>MYKDFANFIRTNKKDLLNNWMNEMEKQSDPLINDIAKEPMYEETSIEFVDLIVSNITENGSKFNEKLDDFAEKVVHLGWPIHFVTTGLRVFGLLVYTAMRDEDLFLKREEKPEDDAYYRFETWLSSMYNKVVTAYADTWEKTVSIQKSALQELSAPLLPIFEKISVMPLIGTIDTERAKLIIENLLIGVVKNRSEVVLIDITGVPVVDTMVAHHIIQASEAVRLVGCQAMLVGIRPEIAQTIVNLGIELDQIITTNTMKKGMERALALTNREIVEKEG[40x];>MGIPILKLGECLLISIQSELDDHTAVEFQEDLLAKIHETSARGVVIDITSIDFIDSFIAKILGDVVSMSKLMGAKVVVTGIQPAVAITLIELGITFSGVLSAMDLESGLEKLKQELGE[20x]

The stressosome is a pseudo-icosahedral megadalton bacterial stress-sensing protein complex consisting of several copies of two STAS-domain proteins, RsbR and RsbS, and the kinase RsbT. Upon perception of environmental stress multiple copies of RsbT are released from the surface of the stressosome. Free RsbT activates downstream proteins to elicit a global cellular response, such as the activation of the general stress response in Gram-positive bacteria. The activation state of the stressosome is reset by the removal of phosphates from RsbS and RsbR by the phosphatase RsbX, allowing for a new round of phosphorylation.

Here, we determined a 3.87 Å reconstruction from a D2 symmetrized cryo-EM map of the stressosome of Listeria innocua (LiRsbRS) assembled from co-expressed LiRsbR and LiRsbS proteins. The stoichiometry of RsbR:RsbS was identical to the one described for the Bacillus stressosome, 20 LiRsbR2:10 LiRsbS2. The 10 LiRsbS dimers form two hook-shaped strips along the core (f in yellow and orange color). A pentameric plane thereby comprises five triangular faces, all of them consisting of one RsbS and two RsbR dimers. LiRsbR enters the STAS domain as the linker helix (ɑ0), while a beta-strand (β0) is found at the N-terminal end in LiRsbS. ɑ3 is well-resolved in LiRsbRS, while it is not resolved in LmRsbR. Interestingly, the MS analysis on the phosphorylation state of the SEC fraction used for structure determination revealed a phosphorylation of Thr241, while conserved sites Thr175 and Thr209 were not phosphorylated. Close to Thr241 in LiRsbR, a spherical density was assigned as phosphoryl group in accordance with the ESI–MS–MS. The phosphoryl-group brings Thr241 in interaction range to Thr209. The superposition of SpoIIAA and LiRsbR revealed that due to the interaction of T209–TPO241, ɑ3 has moved towards ɑ2 in an ‘up-conformation‘ compared to the ɑ3-‘down-conformation‘ in a non-phosphorylated RsbS.>AGHSTQTAEDKEEPLHSIISSTESVQGSTSKHEFQAETKKLLDIVARSLYSEKEVFIRELISNASDALEKLRHKLVSDGQALPEMEIH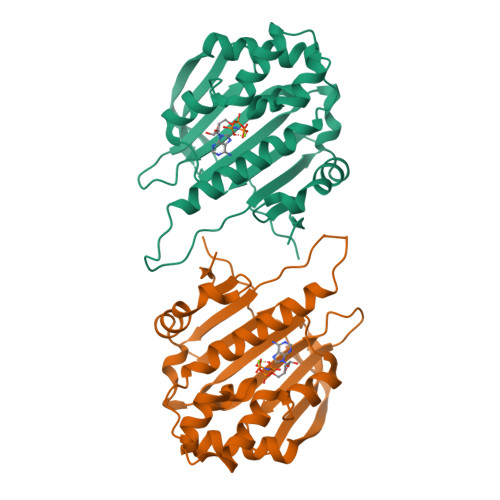LQTNAEKGTITIQDTGIGMTQEELVSNLGTIARSGSKAFLDALQNQAEASSKIIGQFGVGFYSAFMVADRVEVYSRSAAPGSLGYQWLSDGSGVFEIAEASGVRTGTKIIIHLKSDCKEFSSEARVRDVVTKYSNFVSFPLYLNGRRMNT[2x]>[2x]MRSRRVDVMDVMNRLI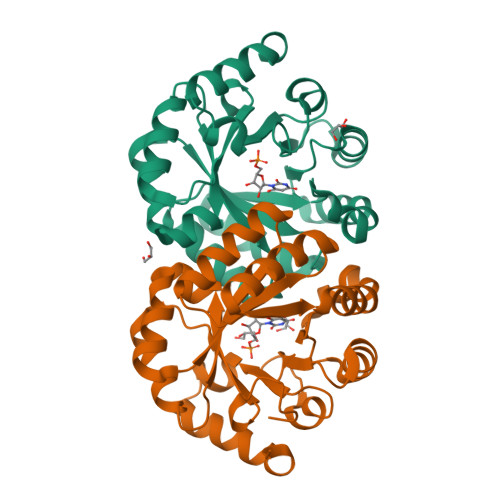LAMDLMNRDDALRVTGEVREYIDTVKIGYPLVLSEGMDIIAEFRKRFGCRIIADFKVADIPETNEKICRATFKAGADAIIVHGFPGADSVRACLNVAEEMGREVFLLTEMSHPGAEMFIQGAADEIARMGVDLGVKNYVGPSTRPERLSRLREIIGQDSFLISPGAGAQGGDPGETLRFADAIIVGASIYLADNPAAAAAGIIESIKDLLNP> MRSSILFLLKLMKIMDVQQQQEAMSSEDRFQELVDSLKPRTAHQYKTYYTKYIQWCQLNQIIPTPEDNSVNSVPYKDLPISAELIHWFLLDTLITDDKPGEKREETEDLDEEEENSFKIATLKKIIGSLNFLSKLCKVHENPNANIDTKYLESVTKLHTHWIDSQKAITTNETNNTNTQVLCPPLLKVSLNLWNPETNHLSEKFFKTCSEKLRFLVDFQLRSYLNLSFEERSKIRFGSLKLGKRDRDAIIYHKVTHSAEKKDTPGHHQLLALLPQDCPFICPQTTLAAYLYLRFYGIPSVSKGDGFPNLNADENGSLLQDIPILRGKSLTTYPREETFSNYYTTVF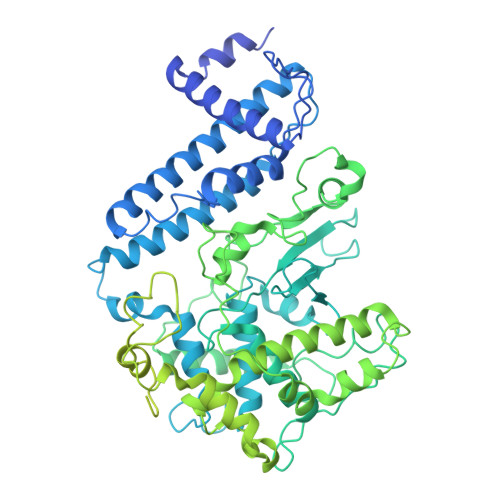RYCHLPYKRREYFNKCNLVYPTWDEDTFRTFFNEENHGNWLEQPEAFAFPDKIPFDFKKIMNFKSPYTSYSTNAKKDPFPPPKDLLVQIFPEIDEYKRHDYEGLSQNSRDFLDLMEVLRERFLSNLPWIYKFFPNHDIFQDPIFGNSDFQSYFNDKTIHSKGSPILSFDILPGFNKIYKNKTNFYSLLIERPSQLTFASSHNPDTHPTQKQESEGPLQMSQLDTTQLNELLKQQSFEYVQFQTLSNFQILLSVFNKIFEKLEMKKSSRGYILHQLNLFKITLDERIKKSKIDDADKFIRDNQPIKKEENIVNEDGPNTSRRTKRPKQIRLLSIADSSDESSTEDSNVFKKDGESIEDGAYGENEDENDSEMQEQLKSMINELINSKISTFLRDQMDQFELKINALLDKILEEKVTRIIEQKLGSHTGKFSTLKRPQLYMTEEHNVGFDMEVPKKLRTSGKYAETVKDNDDHQAMSTTASPSPEQDQEAKSYTDEQEFMLDKSIDSIEGIILEWFTPNAKYANQCVHSMNKSGNKSWRANCEALYKERKSIVEFYIYLVNHESLDRYKAVDICEKLRDQNEGSFSRLAKFLRKWRHDHQNSFDGLLVYLSN> MELKHSISDYTEAEFLQLVTTICNADTSSEEELVKLVTHFAEMTEHPSGSDLIYYPKEGDDDSPSGIVNTVKQWRA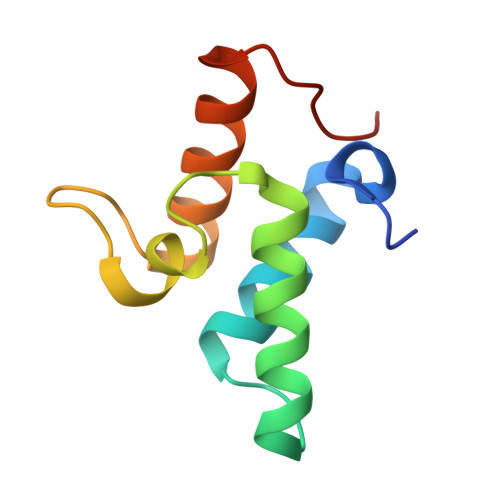ANGKSGFKQG> MLELLPTAVEGVSQAQITGRPEWIW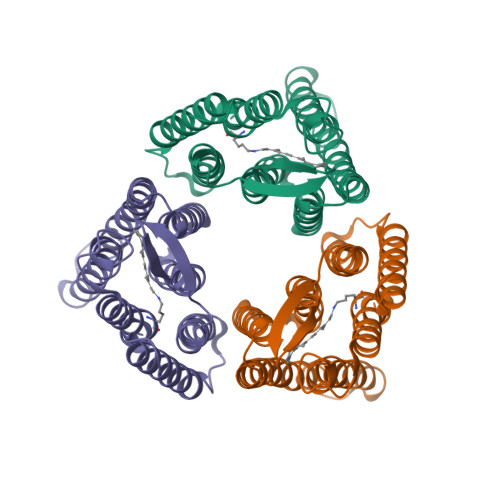LALGTALMGLGTLYFLVKGMGVSDPDAKKFYAITTLVPAIAFTMYLSMLLGYGLTMVPFGGEQNPIYWARYADWLFTTPLLLLDLALLVDADQGTILALVGADGIMIGTGLVGALTKVYSYRFVWWAISTAAMLYILYVLFFGFTSKAESMRPEVASTFKVLRNVTVVLWSAYPVVWLIGSEGAGIVPLNIETLLFMVLDVSAKVGFGLILLRSR>[2x]GSHMTPPHNYLAVIKVVGIGGGGVNAVNRMIEQGLKGVEFIAINTDAQALLMSDADVKLDVGRDSTRGLGAGADPEVGRKAAE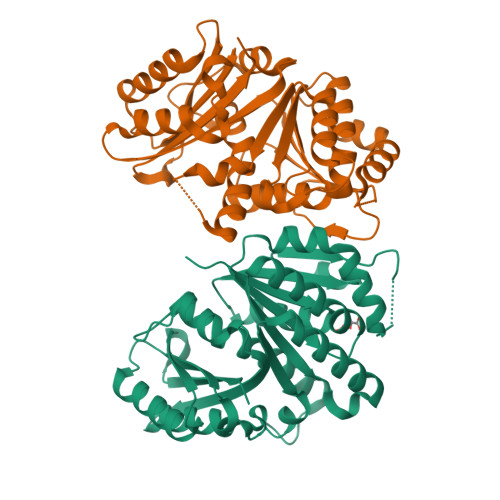DAKDEIEELLRGADMVFVTAGEGGGTGTGGAPVVASIARKLGALTVGVVTRPFSFEGKRRSNQAENGIAALRESCDTLIVIPNDRLLQMGDAAVSLMDAFRSADEVLLNGVQGITDLITTPGLINVDFADVKGIMSGAGTALMGIGSARGEGRSLKAAEIAINSPLLEASMEGAQGVLMSIAGGSDLGLFEINEAASLVQDAAHPDANIIFGTVIDDSLGDEVRVTVIAAGFDVSGPGRKPVMGETGGAHRIESAKAGKLTSTLFEPVDAVSVPLHTNGATLSIGGDDDDVDVPPFMRR> MSPFPLTSMDKAFITVLEMTPVLGTEIINYRDGMGRVLAQDVYAKDNLPPFPASVKDGYAVRAADGPGDRFIIGESQAGEQPTQTVMPGQVMRVTTGAPIPCGADAVVQVEDTELIRESDDGTEELEVRILVQARPGQDIRPIGHDIKRGECVLAKGTHMGPSEIGLLATVGVTEVEVNKFPVVAVMSTGNELLNPEDDLLPGKIRDSNRSTLLATIQEHGYPTINLGIVGDNPDDLLNALNEGISRADVIITSGGVSMGEKDYLKQVLDIDLHAQIHFGRVFMKPGLPTTFATLDIDGVRKIIFALPGNPVSA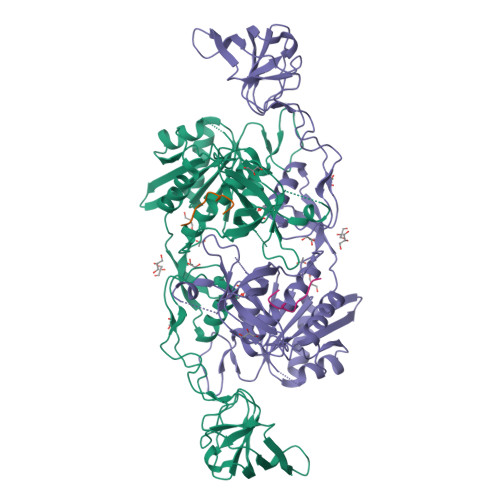VVTCNLFVVPALRKMQGILDPRPTIIKARLSCDVKLDPRPEYHRCILTWHHQEPLPWAQSTGNQMSSRLMSMRSANGLLMLPPKTEQYVELHKGEVVDVMVIGRL;> DFSIVGSLPRDFELS(S)-N-(cyclopentylmethyl)-2-(3-(3,5-difluorophenyl)ureido)-N-(2-(hydroxyamino)-2-oxoethyl)-3,3-dimethylbutanamide 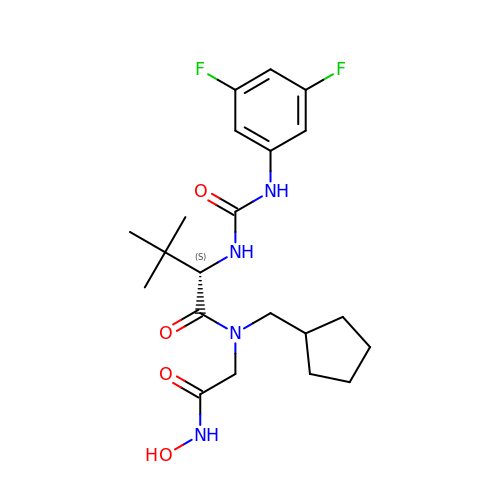| C21 H30 F2 N4 O4 | AJAVBMXPKQJMJH-GOSISDBHSA-N>[2x]PVWGCASTRGRSAEMEDASAAVPR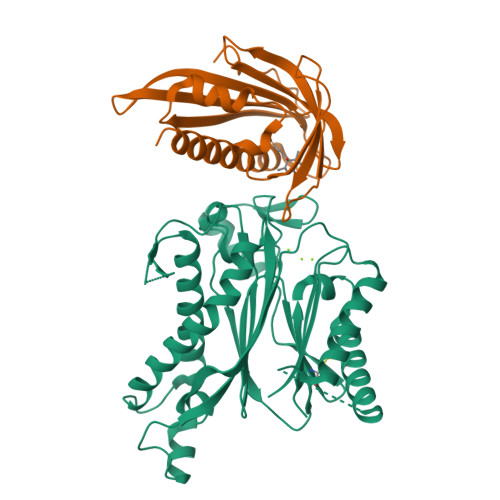FADVPVRLLASRRDLDALGLDADALRLPAHLFGVFDGHGGAEVANYCRERIHVVLSAALARLGKNLGEMGEVDMKEHWDDVFTKCFQRVDDEVSGRVTRVVNGGGEVRSEPVTAENVGSTAVVALVCSSHVVVANCGDSRIVLCRGKEPVALSIDHKPDRKDERARIEAQGGKVIQWNGYRVSGILAMSRSIGDRYLKPFVIPKPEVMVVPRAKDDDCLILASDGLWDVVSNEEACKVARRQILLWHKNNGAASPLSDEGEGSTDPAAQAAADYLMRLALKKGSEDNITVIVVDLKPRKKLKN;>[2x]ETEYVRRFHRHEPRDHQCSSAVAKHIKAPVHLVWSLVRRFDQPQLFKPFVSRCEMKGNIEIGSVREVNVKSGLPATRSTERLELLDDNEHILSVRFVGGDHRLKNYSSILTVHPEVIDGRPGTLVIESFVVDVPEGNTKDETCYFVEALLKCNLKSLAEVSERLVVKDQTEPLDR>[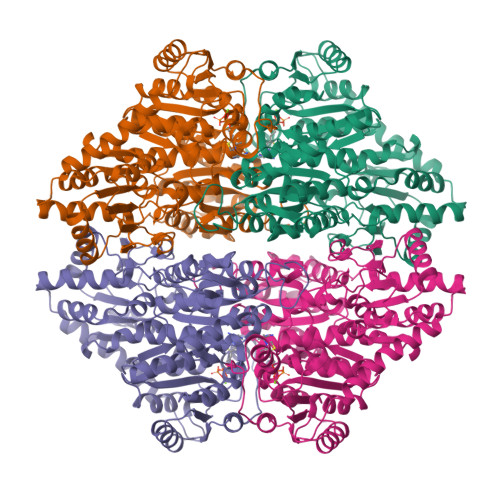4x]MAMITGGELVVRTLIKAGVEHLFGLHGAHIDTIFQACLDHDVPIIDTRHEAAAGHAAEGYARAGAKLGVALVTAGGGFTNAVTPIANAWLDRTPVLFLTGSGALRDDETNTLQAGIDQVAMAAPITKWAHRVMATEHIPRLVMQAIRAALSAPRGPVLLDLPWDILMNQIDEDSVIIPDLVLSAHGARPDPADLDQALALLRKAERPVIVLGSEASRTARKTALSAFVAATGVPVFADYEGLSMLSGLPDAMRGGLVQNLYSFAKADAAPDLVLMLGARFGLNTGHGSGQLIPHSAQVIQVDPDACELGRLQGIALGIVADVGGTIEALAQATAQDAAWPDRGDWCAKVTDLAQERYASIAAKSSSEHALHPFHASQVIAKHVDAGVTVVADGALTYLWLSEVMSRVKPGGFLCHGYLGSMGVGFGTALGAQVADLEAGRRTILVTGDGSVGYSIGEFDTLVRKQLPLIVIIMNNQSWGATLHFQQLAVGPNRVTGTRLENGSYHGVAAAFGADGYHVDSVESFSAALAQALAHNRPACINVAVALDPIPPEELILIGMDPFA PfEMP1s are adhesive proteins containing multiple discrete extracellular domains, falling mostly into two families, the cysteine-rich interdomain region and the Duffy binding-like (DBL) domains. While several DBL domains from different PfEMP1 proteins bind to CSA, VAR2CSA is the primary CSA receptor in placental malaria. The binding of VAR2CSA on the surface of infected erythrocytes to CSPG in the placenta plays a major part in malaria during pregnancy, and an understanding of this interaction will be valuable in the development of therapeutics to target this form of the disease. In this study, we present the structure of the DBL6ɛ domain of VAR2CSA and characterisation of the CSPG-binding sites of the DBL3X and DBL6ɛ domains.

Using a bacterial expression system, we expressed the DBL6ɛ domain of VAR2CSA (residues 2333–2634) from the 3D7 strain of Plasmodium falciparum. We expressed both the DBL6ɛ domain and the C2480S mutant and were able to crystallise C2480S. The structure was determined using multiple-wavelength dispersion data from a selenomethionine derivative and was refined to 3.0 Å resolution. DBL6ɛ shares a similar basic fold with other DBL domains containing a “boomerang”-shaped α-helical core that aligns to the core of the DBL3X structure with a root-mean-square deviation of 1.6 Å. DBL6ɛ is shorter (302 residues compared with 359 for DBL3X) due to more compact loop structures and a shorter subdomain 1. DBL6ɛ also contains fewer disulfide bonds than other DBL domain structures, lacking three of the bonds that stabilise the first two subdomains of DBL3X. While all other current DBL domain structures contain a disulfide bond linking the second helix of subdomain 2 to the linker that connects subdomains 2 and 3, this is not present in DBL6ɛ, showing that this bond is not essential for the DBL domain fold. Indeed, the features proposed to form the CSPG-binding site of DBL3X, the sulfate-binding loop and the positively charged surface, are absent in DBL6ɛ, agreeing with a recent prediction based on molecular modeling. However, no clear additional density due to ligand could be observed after structure determination.

>ICNKYKNINVNMKKNNDDTWTDLVKNSSDINKGVLLPPRRKNLFLKIDESDICKYKRDPKLFKDFIYSSAISEVERLKKVYGEAKTKVVHAMKYSFADIGSIIKGDDMMENNSSDKIGKILGDGVGQNEKRKKWWDMNKYHIWESMLSGYKHAYGNISENDRKMLDIPNNDDEHQFLRWFQEWTENFCTKRNELYENMVTACNSAKCNTSNGSVDKKECTEACKNYSNFILIKKKEYQSLNSQYDMNYKETKAEKKESPEYFKDKCNGECSCLSEYFKDETRWKNPYETLDDTEVKNNCMCK[2x]3-[(E)-2-(2-chloro-4-{[3-(2,6-dichlorophenyl)-5-(1-methylethyl)isoxazol-4-yl]methoxy}phenyl)ethenyl]benzoic 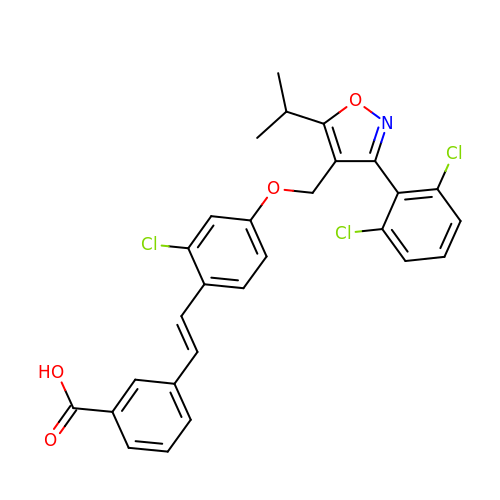acid | C28 H22 Cl3 N O4 | BYTNEISLBIENSA-MDZDMXLPSA-N>GMSEPQRLFFAIDLPAEIREQIIHWRAKHFPPEAGRPVAADNLHLTLAFLGEVSAEKEKALSLLAGRIRQPGFTLTLDDAGQWLRSRVVWLGMRQPPRGLIQLANMLRSQAARSGCFQSNRPFHPHITLLRDASEAVTIPPPGFNWSYAVTEFTLYASSFARGRT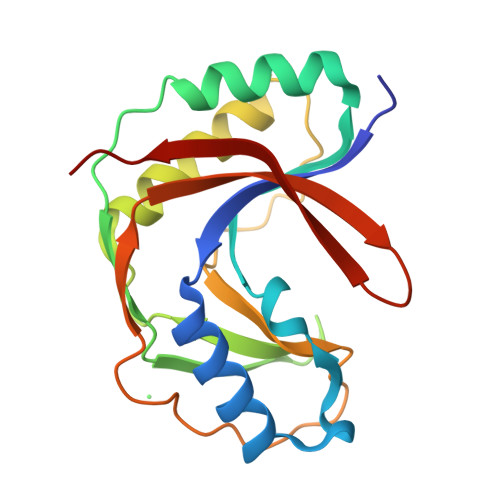RYTPLKRWALTQ[4x]>[2x]GMVRISIAGGNEIDPGSMGLTLFHEHLRLITEVVRWNWPHLYNEDEELKRAIDAVNAAKKYGVKTIIDLTVAGIGCDVRFNEKVAKATGVNIIMGTGFYTYTEIPFYFKNRGIDSLVDAFVHDITIGIQGTNTRAAFVKAVIDSSGLTKDVEMAIRAAAKAHIKTDVPIITHSFVGNKSSLDLIRIFKEEGVDLARTVIGHVGDTDDISFIEQILREGAFIGLDRFGLDIYLPLDKRVKTAIELIKRGWIDQLLLSHDYCPTIDWYPPEVVRSTVPDWTMTLIFEKVIPRMRSEGITEEQINRVLIDNPRRLFTGR

VmoLac (YP_004245953) is a recently identified enzyme that was isolated from the hyperthermophilic crenarchaeon Vulcanisaeta moutnovskia strain 768-2833. The phylogenetic tree that was built from this sequence alignment, indicates that VmoLac belongs to the clade of the PLLs-A. Kinetic characterization indicates that VmoLac is a proficient lactonase with promiscuous, poor esterase and phosphotriesterase activities. As expected, VmoLac is roughly globular and exhibits a (β/α)8 barrel topology that is similar to that of others PLLs such as SsoPox17, SisLac8, DrOPH3, GsP10 and GkL36.

Interestingly, VmoLac was crystallized in two different space groups. The structure that was solved in P64 reveals a homodimer in the asymmetric unit, as previously observed for other PLLs, such as SsoPox. A clear extra density was observed in the active sites of both of the VmoLac structures, although no potential substrates were present in the crystallization conditions. Because of a relatively good resolution of the structures (1.8 and 2.35 Å), this unexpected density could be attributed to a fatty acid with good confidence. However, the precise nature of this fatty acid is uncertain: the number of carbon atoms is clear from the electronic density maps, but possible unsaturation is difficult to interpret from density maps. Therefore, this density was attributed to the simplest fatty acid that fit the observed density and that was present in the expression host E. coli: myristic acid. The carboxylate of the fatty acid molecule is tightly bound to the bi-metallic active site (2.2 Åα–2.3 Åβ), while the long aliphatic fatty chain that sits in the hydrophobic channel is mainly formed by loop 8 residues. Notably, the bound fatty acid adopts a slightly different binding mode in both of the monomers, and movements of residues on the active site loop 7 can be observed (Ile229 and Tyr230). As expected, both of the structures are nearly identical (r.m.s.d for α-carbon atoms (over 315 atoms) of 0.34 Å), but some slight differences can be observed in the active site region (loops 7 and 8). In particular, loop 8 residues Y265, V269, V270 and T273 occupy slightly altered conformations, whereas loop 7 undergoes a larger conformational displacement.[(1R)-1-[[(2S)-2-methyl-3-sulfanyl-propanoyl]amino]-2-phenyl-ethyl]boronic acid | C12 H18 B N O3 S | 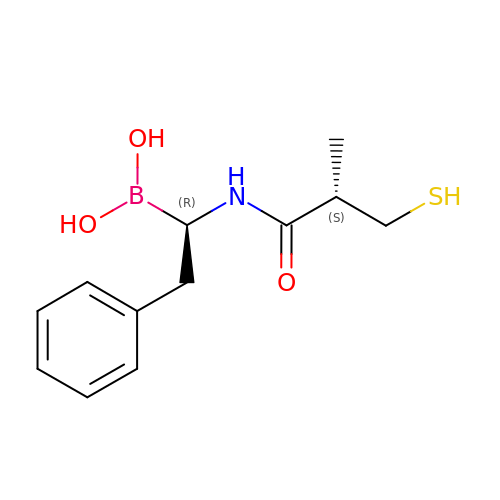FYDJFEUAPCQUQY-KOLCDFICSA-N> MAEGEITTFTALTEKFNLPPGNYKKPKLLYCSNGGHFLRILPDGTVDGTRDRSDQHIQLQLSAESVGEVYIKSTETGQYLAMDTDGLLYGSQTPNEECLFLERLEENHYNTYISKKHAEKNWFVGLKKNGSCKRGPRTHYGQKAILFLPLPVSSD;> MGRAAEVPGPEPGQQEQLVFGSGDAVELSCPPPGGGPMGPTVWVKDGTGLVPSERVLVGPQRLQVLNASHEDSGAYSCRQRLTQRVLCHFSVRVTDAPSSGDDEDGEDEAEDTGVDTGAPYWTRPERMDKKLLAVPAANTVRFRCPAAGNPTPSISWLKNGREFRGEHRIGGIKLRHQ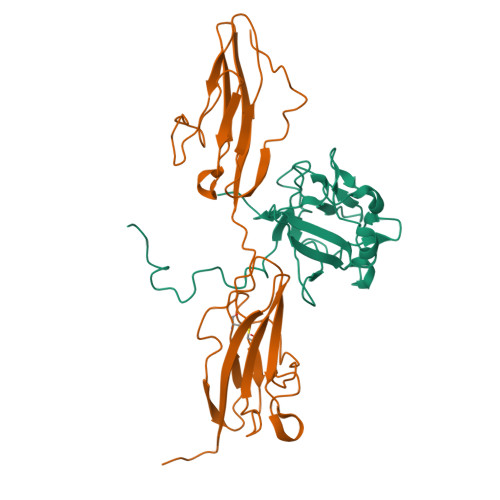QWSLVMESVVPSDRGNYTCVVENKFGSIRQTYTLDVLERSPHRPILQAGLPANQTAVLGSDVEFHCKVYSDAQPHIQWLKHVEVNGSKVGPDGTPYVTVLKTAGANTTDKELEVLSLHNVTFEDAGEYTCLAGNSIGFSHHSAWLVVLPAEEELVE>[2x]MGVDPFERNKILGRGINIGNALEAPNEGDWGVVIKDEFFDIIKEAGF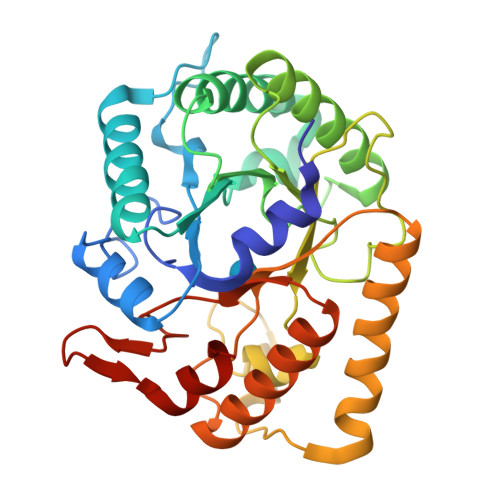SHVRIPIRWSTHAYAFPPYKIMDRFFKRVDEVINGALKRGLAVVINIHHYEELMNDPEEHKERFLALWKQIADRYKDYPETLFFEILNAPHGNLTPEKWNELLEEALKVIRSIDKKHTIIIGTAEWGGISALEKLSVPKWEKNSIVTIHYYNPFEFTHQGAEWVEGSEKWLGRKWGSPDDQKHLIEEFNFIEEWSKKNKRPIYIGEFGAYRKADLESRIKWTSFVVREMEKRRWSWAYWEFCSGFGVYDTLRKTWNKDLLEALIGGDSIE> LTGQIDRALESIHGTDEAEALAVAN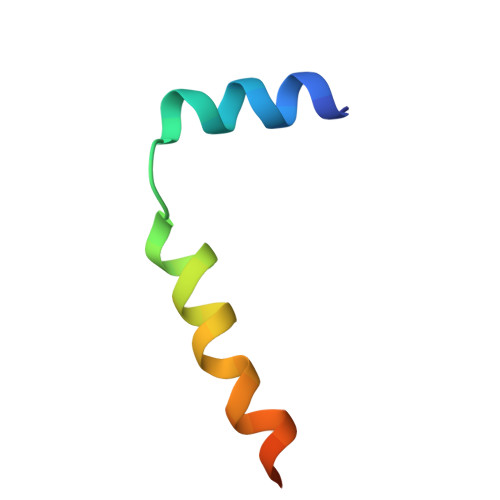AYRVLETMDDEW>GGGGMLTLIQGKKIVNHLRSRLAFEYNGQLIKILSKNIVAVGSLRREEKMLNDVDLLIIVPEKKLLKHVLPNIRIKGLSFSVKVCGERKCVLFIEWEKKTYQLDLFTALAEEKPYAIFHFTGPVSYLIRIRAALKKKNYKLNQYGLFKNQTLVPLKITTEKELIKELGFTYRIPKKRL[2x]

To provide a molecular basis for designing better drugs targeting polymerases, African swine fever virus DNA Polymerase X (Pol X) was used as a model for the study. As the simplest DNA polymerase identified to date, Pol X belongs to the polymerase X family and is constituted of 174 amino acids. In this chemical reaction, metal-ion A (MeA) is a catalytic ion and decreases the pKa of 3′-OH, facilitating its attack on the α-phosphate of the incoming dNTP, and metal-ion B (MeB) stabilizes the dNTP-DNA-polymerase complex and increases the electrophilicity of the phosphorus center. To clearly understand the phosphodiester-bond-formation mechanism and the metal-ion catalysis of polymerases, we designed modified dNTP substrates with a chiral α-phosphorus center (α-P center) using a single selenium atom, without affecting the overall and local structures, to explore the absolute configuration inversion and probe the mechanisms of the metal ion–oxygen interactions.

DNApre, generated on the DNA-I by incorporating ddNTP without 3′-OH, failed to attack the incoming dNTP (dGTP, dGTPαSe-I, or dGTPαSe-II), thereby forming the substrate complex (the substrate–primer-template–polymerase complex: nat-dG_sub, dGSe-I_sub, or dGSe-II_sub), resulting in the before-reaction state (without the bond formation) retaining the absolute configuration of dGTPαSe. In crystallization trials, DNApre-I (generated form 5′-CAGGATCCT-3′ with ddTTP, without 3′-OH) and DNApre-II (generated form 5′-CTGGATCCA-3′ with ddATP, without 3′-OH) could not be extended by attacking dGTP or dGTPαSe diastereomers in the crystallization conditions, which allowed the dNTPs to just bind and retain their absolute configuration. Firstly, dGTPαSe diastereomers were synthesized and separated by reversed-phase-HPLC as peak 1 (dGTPαSe-I, eluted first on HPLC) and peak 2 (dGTPαSe-II, eluted later), and their absolute configurations on the α-P center were determined as Rp and Sp, respectively, by X-ray crystallography. The nat-dG_sub and dGSe-II_sub structures were refined at similar resolutions, 2.25 and 2.29 Å, respectively. However, when comparing the substrate structures containing native dGTP and dGTPαSe-II, we only found a strong Se-density difference in the electron map, which indicated the Sp configuration on the Se-modified α-P center, determining the absolute configuration of dGTPαSe-II (Sp diastereomer). As expected, all structures of the three substrate complexes captured the reaction state at the pre-polymerization level, and they belonged to the P212121 space group. Superposition showed that the three overall structures were very similar, and their root-mean-square deviations (RMSD) were approximately 0.7–1.3 Å.> MAVVLPDWYEEAFVNVENLFIDMFTDLLPDYESGCWAPDDWLADEIEVKPTIWFFRLPGGR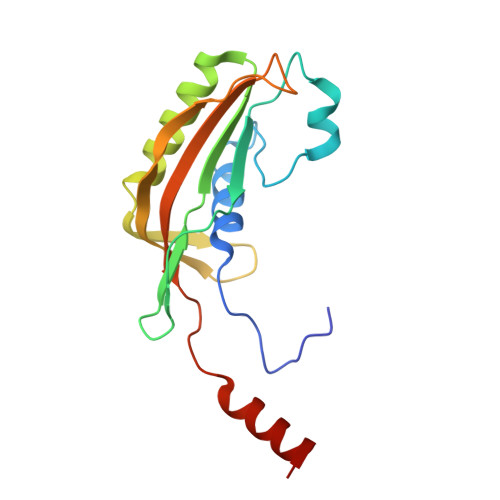VDWDGRKDECQLQVMVVTGSRDDSWRLMDFVRAMLLPMQGDKYKMADGYTAQIRCAGEVAGPQLLTPGQRIDTRVVTATFKVSVSMKSAKNYKQKLYELWQALRGS> GSYNRLQQDILEPFERALKLQTVS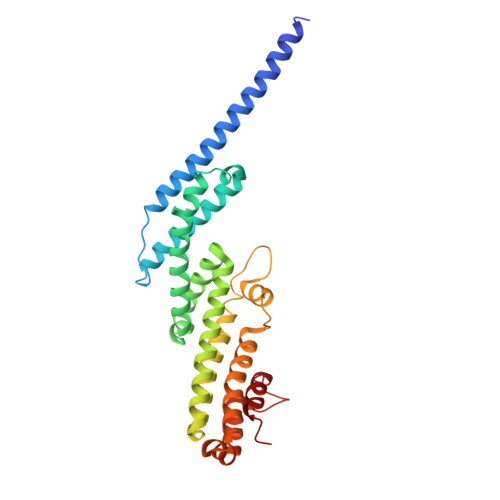SKIHQTTTLLRSSLIYVHMISQLQMMPLETDSTDDAALACGLKIAALHSQLKINIAANPNLATLQLIKSCENNVVSPNRQELLRYLSTNLTRDCLNNLKMENNPKRIVTLIKALYTLSPVDLFDTIDKVLSSKIQTTAQVLSKTITSIRNFNLSLDDAMENRNSILTLQNLMAACAIEGNTNTLRNYLSQRKFSSLIDQFWSKVTNSFKRDFEMSYNRGGPVGKSLQSNSNLIYEAISKCFGENDPSNELQGELQYILKAVSILDT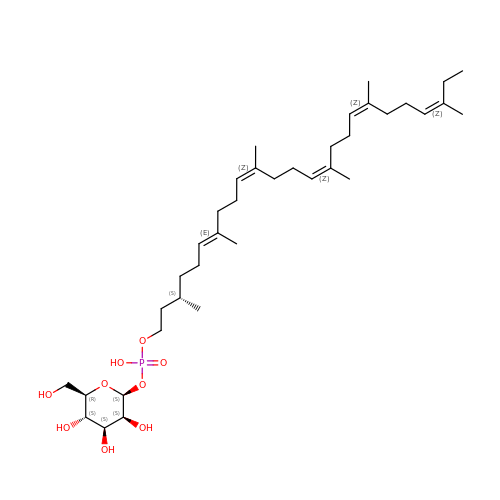dolichol-phosphate-mannose (n=2) | C37 H65 O9 P | RYYUUUNCYTWVRE-OGASEETLSA-N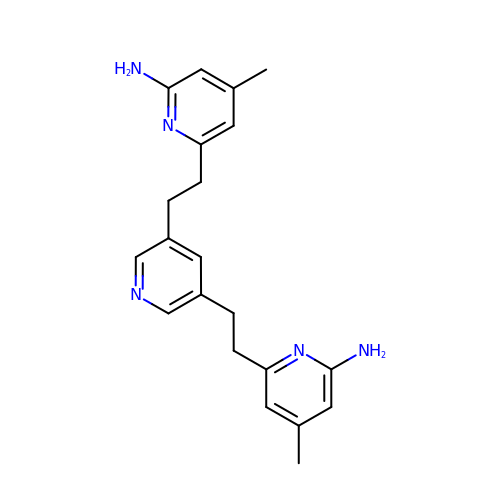6,6'-(pyridine-3,5-diyldiethane-2,1-diyl)bis(4-methylpyridin-2-amine) | C21 H25 N5 | KZHFSPGMRFCRCE-UHFFFAOYSA-N>[2x]KPTVKEIKSLQNFNRIAGVFHLLQMLAVLALANDFALPMTGTYLNGPPGTTFSAPVVILETPVGLAVALFLGLSALFHFI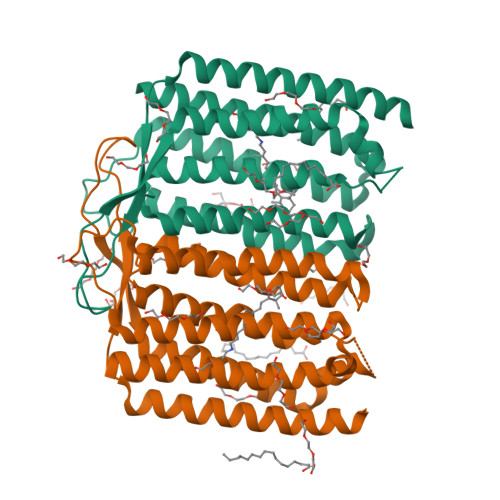VSSGNFFKRYSASLMKNQNIFRWVEYSLSSSVMIVLIAQICGIADIVALLAIFGVNASMILFGWLQEKYTQPKDGDLLPFWFGCIAGIVPWIGLLIYVIAPGSTSDVAVPGFVYGIIISLFLFFNSFALVQYLQYKGKGKWSNYLRGERAYIVLSLVAKSALAWQIFSGTLI>GPLGSDLKDAEAVQKFFLEEIQLGEELLAQGDYEKGVDHL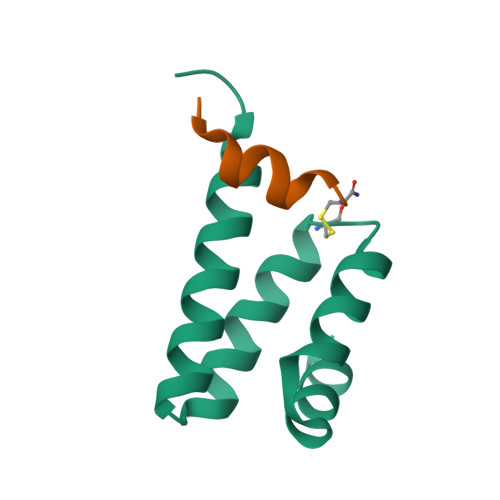TNAIAVCGQPQQLLQVLQQTLPPPVFQMLLTKL[7x];>GPRLSRLLSYAGC[7x]(1R)-3-amino-1-{4-fluoro-3-[(2-propylpentyl)oxy]phenyl}propan-1-ol 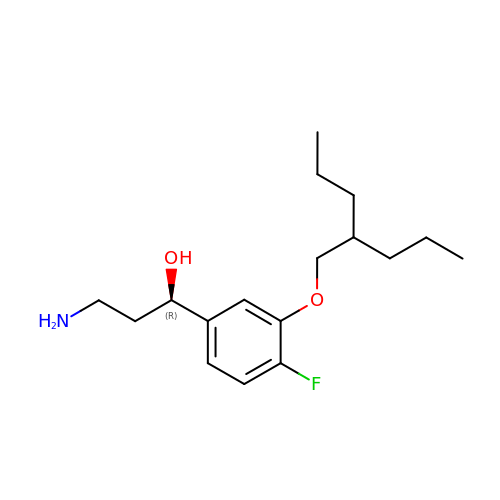| C17 H28 F N O2 | WDYVEMOTVIKKNU-MRXNPFEDSA-N> MKYMITSKGDEKSDLLRLNMIAGFGEYDMEYDDVEPEIVISIGGNGTFLSAFHQYEERLDEIAFIGIHTGHLGFYADWRPAEADKLVKLLAKGEYQKVSYPLLKTTVKYGIG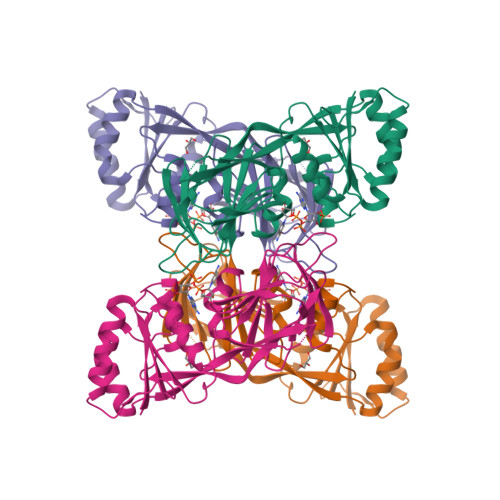KKEATYLALNESTVKSSGGPFVVDVVINDIHFERFRGDGLCMSTPSGTTAYNKSLGGALMHPSIEAMQLTEMASINNRVYRTIGSPLVFPKHHVVSLQPVNDKDFQISVDHLSILHRDVQEIRYEVSAKKIHFARFRSFPFWRRVHDSFIEDLEHHHHHH>XXXXXXXXXXXXEEQRRKKRRLKKRIFAAVSEGCVEELVELLVELQELCRRRHDEDVPDFLMHKLTASDTGATCLMKALLNINPNTKEIVRILLAFAEENDILGRFINAEYTEEAYEGQTALNIAIERRQGDIAALLIAAGADVNAHAKGAFFNPKYQHEGFYFGETPLALAACTNQPEIVQLLMEHEQTDITSRDSRGNNILHALVTVAEDFKTQNDFVKRMYDMILLRSGNWELETTRNNDGLTPLQLAAKMGKAEILKYILSREIKEKRLRSLSRKFTDWAYGPVSSSLYDLTNVDTTTDNSVLEITVYNTNIDNRHEMLTLEPLHTLLHMKWKKFAKHMFFLSFCFYFFYNITLTLVSYYRPREEEAIPHPLALTHKMGWLQLLGRMFVLIWAMCISVKEGIAIFLLRPSDLQSILSDAWFHFVFFIQAVLVILSVFLYLFAYKEYLACLVLAMALGWANMLYYTRGFQSMGMYSVMIQKVILHDVLKFLFVYIVFLLGFGVALASLIEKCPKDNKDCSSYGSFSDAVLELFKLTIGLGDLNIQQNSKYPILFLFLLITYVILTFVLLLNMLIALMGETVENVSKESERIWRLQRARTILEFEKMLPEWLRSRFRMGELCKVAEDDFRLCLRINEVKWTEWKTHVSFLNEDPGPVRRTDFNKIQDSSRNNSKTTLNAFEEVEEFPETSVVDAGLEVLFQGDYKDDDDKAH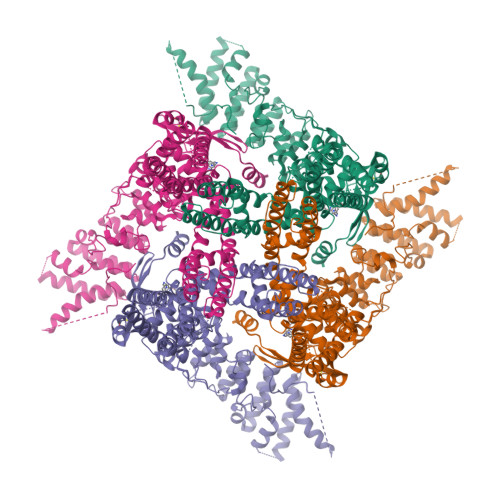HHHHH[4x]> AGAGADRTAATPAAANPAATEPVKWECPAGYEVKEGLNVDFPHKGMKRAFIVYPAKNVSGPAPVWVPMTGSVESTNDNLTVARSGANSILADHGYTVIAPVRACANQDPNIRGERCNGPGSNGWNWNPWFEGRAADPSGEHWKNDEGPDSSFFVAMVQCVGTKY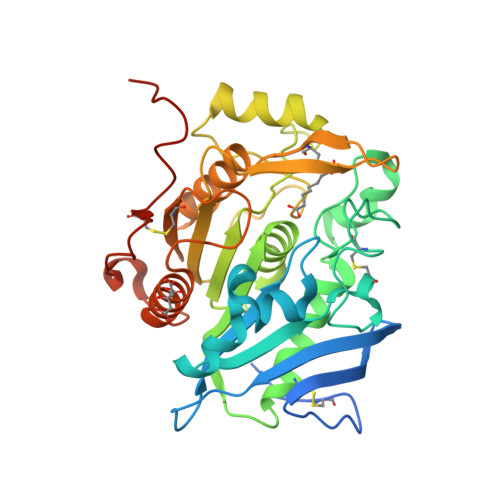KLDARRLFLGGIASGGTMTNRALLFRSNFWAGGLPISGEWYVTSDDGTPLSFDDARAAVAAAPTKIHQGRVGPYPLPAKVGPLIVMTVWGGEKDLWNCTRPDGSRFLCADYRPSTQAGSNFFSAQPDVVHVACSSTHGHMWPQLNTQEFNRWALDTLASHPKGSDPRSFKLTQPPEGYTCHVGPFTGLYASAWSHPQFEK>[2x]AGAGAMYDIKKWRHIFKLDPAKHISDDDLDAICMSQTDAIMIGGTDD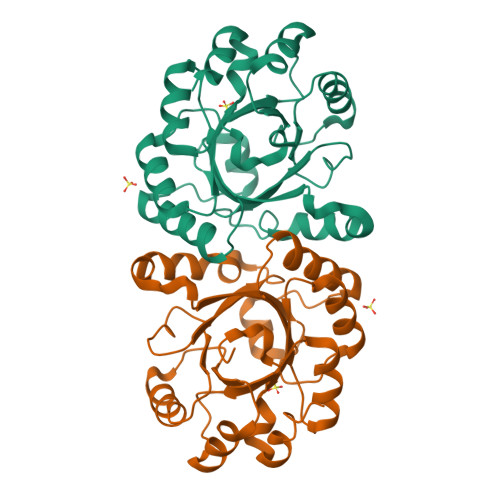VTEDNVIHLMSKIRRYPLPLVLEISNIESVMPGFDFYFVPTVLNSTDVAFHNGTLLEALKTYGHSIDFEEVIFEGYVVCNADSKVAKHTKANTDLTTEDLEAYAQMVNHMYRLPVMYIEYSGIYGDVSKVQAVSEHLTETQLFYGGGISSEQQATEMAAIADTIIVGDIIYKDIKKALKTVKIKESSK> MSHHHHHHSMQRTKIVVKVHMPCGKSRAKALALAASV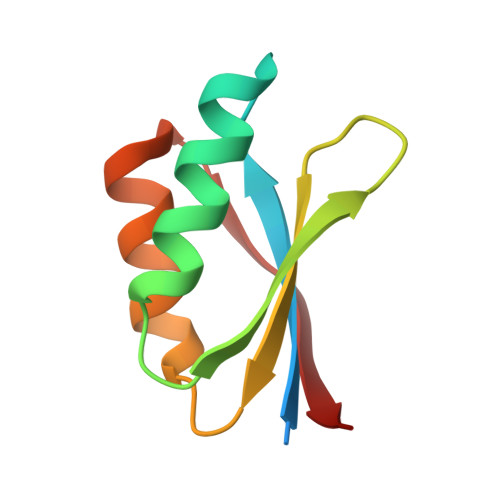NGVDSVEITGEDKDRLVVVGRGIDPVRLVALLREKCGLAELLMVELV>GVTLLLPEPEWTYPRLSCPGSTFQKALLISPHRFGETKGNSAPLIIREPFIACGPKECKHFALTHYAAQPGGYYNGTRGDRNKLRHLISVKLGKIPTVENSIFHMAAWSGSACHDGKEWTYIGVDGPENNALLKIKYGEAYTDTYHSYANNILRTQESACNCIGGNCYLMITDGSASGISECRFLKIREGRIIKEIFPTGRVKHTEECTCGFASNKTIECACRDNSYTAKRPFVKLNVETDTAEIRLMCTETYLDTPRPDDGSITGPCESNGDKGSGGIKGGFVHQRMASKIGRWYSRTMSKTKRMGMGLYVKYDGDPWTDSDALALSGVMVSMEEPGWYSFGFEIKDKKCDVPCIGIEMVHDGGKET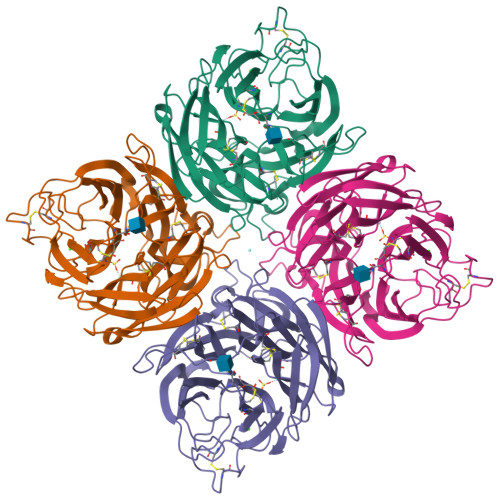WHSAATAIYCLMGSGQLLWDTVTGVDMAL[16x]>[3x]MKIEEVKSTTKTQRIASHSHVKGLGLDESGLAKQAASGLVGQENAREACGVIVELIKSKKMAGRAVLLAGPPGTGKTALALAIAQELGSKVPFCPMVGSEVYSTEIKKTEVL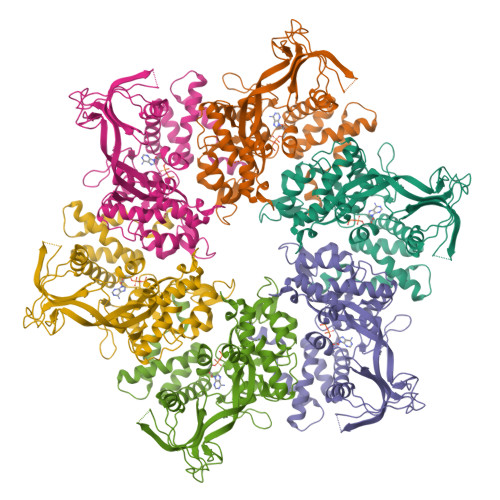MENFRRAIGLRIKETKEVYEGEVTELTPCETENPMGGYGKTISHVIIGLKTAKGTKQLKLDPSIFESLQKERVEAGDVIYIEANSGAVKRQGRCDTYATEFDLEAEEYVPLPKGDVHKKKEIIQDVTLHDLDVANARPQGGQDILSMMGQLMKPKKTEITDKLRGEINKVVNKYIDQGIAELVPGVLFVDEVHMLDIECFTYLHRALESSIAPIVIFASNRGNCVIRGTEDITSPHGIPLDLLDRVMIIRTMLYTPQEMKQIIKIRAQTEGINISEEALNHLGEIGTKTTLRYSVQLLTPANLLAKINGKDSIEKEHVEEISELFYDAKSSAKILADQQDKYMK> MIIPALNLIDGTVVRLHQGDYARQRDYGNDPLPRLQDYAAQGAGVLHLVDLTGAKDPAKRQIPLIKTLVAGVNVPVQVGGGVRTEEDVAALLKAGVARVVIASTAMKSPDVVKGWFERFGAQALVLALDVRIDEHGTKQVAVSGWQENSGVSLEQLVETYLPVGLKHVLCTDISRAGTLAGSNVSLYEEVCARYPQI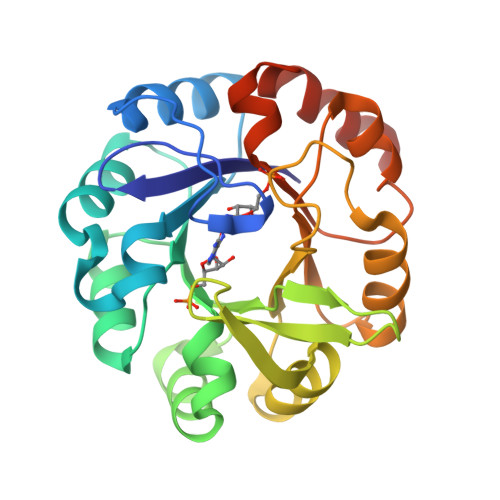AFQSSGGIGDIDDIAALRGTGVRGVIVGRALLEGKFTVKEAIQCWQNVKGHHHHHH> DYWKPRHHPPRNN;> CNWTGVKCNRRGEVSEIQLKEKQLQGSLPVTSLRSLKSLTSLTLSSLQLTGVIPKEIGDFTELELLDLSDNSLSGDIPVEIFRLKKLKTLSLNTNNLEGHIPMEIGNLSGLVELMLFDNKLSGEIPRSIGELKNLQVLRAGGNKNLRGELPWEIGNCENLVMLGLAETSLSGKLPASIGNLKRVQTIAIYTSLLSGPIPDEIGYCTELQNLYLYQNSISGSIPTTIGGLKKLQSLLLWQNNLVGKIPTELGNCPELWLIDFSENLLTGTIPRSFGKLENLQELQLSVNQISGTIPEELTNCTKLTHLEIDNNLITGEIPSLMSNLRSL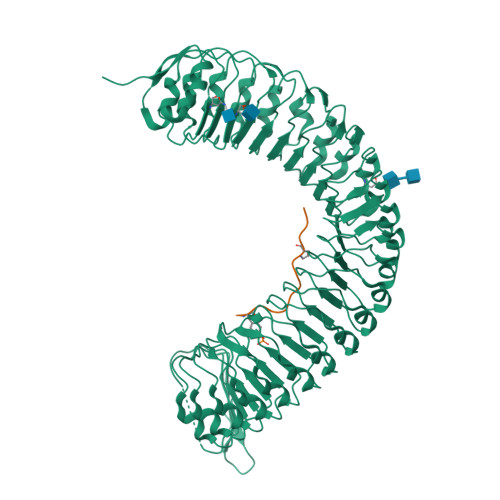TMFFAWQNKLTGNIPQSLSQCRELQAIDLSYNSLSGSIPKEIFGLRNLTKLLLLSNDLSGFIPPDIGNCTNLYRLRLNGNRLAGSIPSEIGNLKNLNFVDISENRLVGSIPPAISGCESLEFLDLHTNSLSGSLLGTTLPKSLKFIDFSDNALSSTLPPGIGLLTELTKLNLAKNRLSGEIPREISTCRSLQLLNLGENDFSGEIPDELGQIPSLAISLNLSCNRFVGEIPSRFSDLKNLGVLDVSHNQLTGNLNVLTDLQNLVSLNISYNDFSGDLPNTPFFRRLPLSDLASNRGLYISNAIST>[2x]MIKRYLQFVKPYKYRIFATIIVGIIKFGIPMLIPLLIKYAIDGVINNHALTTDEKVHHLTIAIGIALFIFVIVRPPIEFIRQYLAQWTSNKILYDIRKKLYNHLQALSARFYANNQVGQVISRVINDVEQTKDFILTGLMNIWLDCITIIIALSIMFFLDVKLTLAALFIFPFYILTVYVFFGRLRKLTRERSQALAEVQGFLHERVQGISVVKSFAIEDNEAKNFDKKNTNFLTRALKHTRWNAY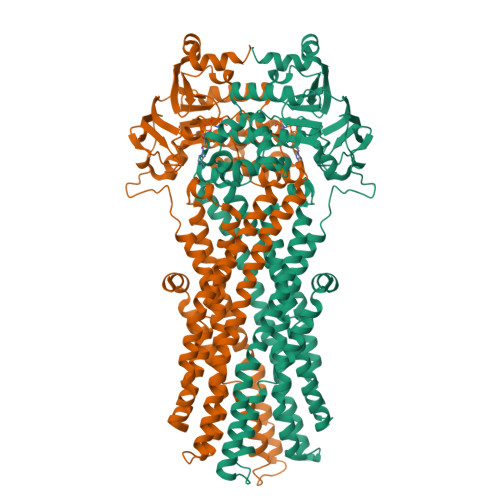SFAAINTVTDIGPIIVIGVGAYLAISGSITVGTLAAFVGYLELLFGPLRRLVASFTTLTQSFASMDRVFQLIDEDYDIKNGVGAQPIEIKQGRIDIDHVSFQYNDNEAPILKDINLSIEKGETVAFVGMSGGGKSTLINLIPRFYDVTSGQILIDGHNIKDFLTGSLRNQIGLVQQDNILFSDTVKENILLGRPTATDEEVVEAAKMANAHDFIMNLPQGYDTEVGERGVKLSGGQKQRLSIARIFLNNPPILILDEATSALDLESESIIQEALDVLSKDRTTLIVAHRLSTITHADKIVVIENGHIVETGTHRELIAKQGAYEHLYSIQNL>[2x]AHHHHHHGE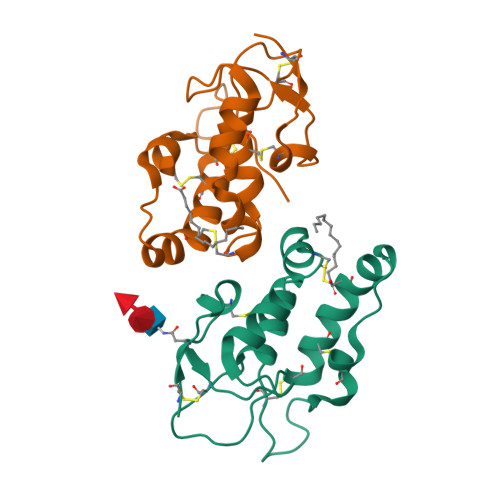NLYFQGSKAPVCQEITVPMCRGIGYNLTHMPNQFNHDTQDEAGLEVHQFWPLVEIQCSPDLRFFLCSMYTPICLPDYHKPLPPCRSVCERAKAGCSPLMRQYGFAWPERMSCDRLPVLGRDAEVLCMDYERSEAGNS(12R)-12-methyltetradecanoic 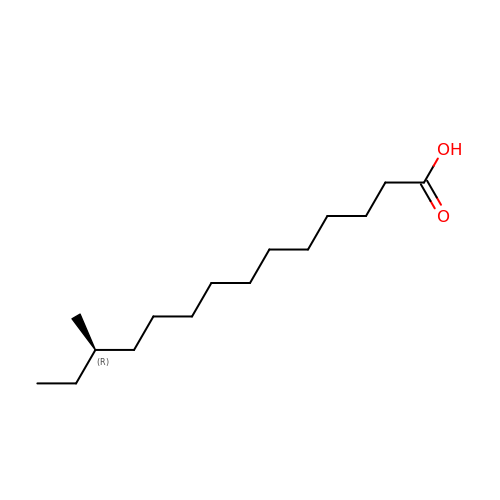acid | C15 H30 O2 | XKLJLHAPJBUBNL-CQSZACIVSA-N> MGSSHHHHHHENLYFQGSMKEQLKPLLEDKTYLRHFWHPVCTLNEFERANASGHGPMGVTLLGEKLVLARLNSKIIAAADRCAHRSAQLSIGRVCSNAGKDYLECPYHGWRYDEAGACQLIPACPDKSISPRAKISSFDCEVKYDIV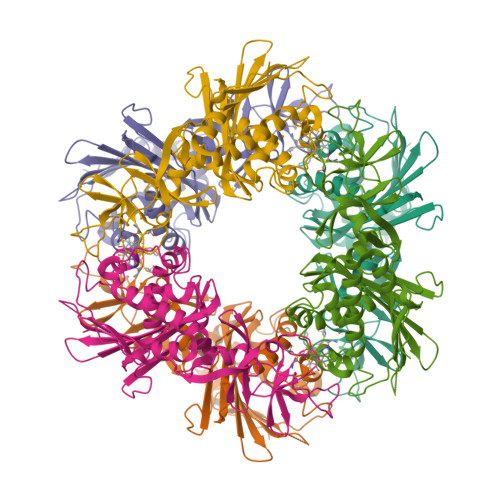WVRLDNSFDCTQIPYLSDFDNPDMQVIVADSYIWETVAERRWENFTDFSHFAFVHPGTLYDPFFASHPTVYVNRVDGELQFKLAPPREMKGIPPEAPMGDFTYRCTMPYSVNLEIKLWKDDSRFVLWTTASPVDNKSCRNFMIIVREKDNQPDHMHLAFQKRVLDEDQPVIESQWPLEIQTSEVSVATDKISVQFRKWHKELSLSAVEGREAFRDSVLTNVIEEEQ In this work, a novel β‐glucosidase (WP_026963033.1) of the glycosyl hydrolase family 1 (GH1) from the extremophilic organism Alicyclobacillus herbarius (Ahe) has been identified and investigated. β‐Glucosidases (EC 3.2.1.21) constitute a group of enzymes that hydrolyse terminal, non‐reducing glycosyl residues from glycosides. AheGH1 is arranged into a single (β/α)8 barrel fold, common to this family of glycosidases, with negligible main‐chain displacements in peripheral loops and α‐helices. As a particular example, the evaluation of the hydrolytic capacity of AheGH1 towards the most common isoflavone glucosides found in soybeans, concluded that the enzyme can efficiently convert isoflavone glucosides into aglycones, and hence, it constitutes a promising candidate for the enzymatic production of soybean isoflavones.

Crystals of AheGH1 enzyme belonging to the monoclinic space group P21 diffracted at 1.98 Å resolution. The asymmetric unit of AheGH1 contains four independent molecules, with a calculated Matthews coefficient of 2.42 Å3 Da1 (estimated solvent content of 49.31 %). The overall structure of the four AheGH1 subunits is identical (RMSD values of 0.05 to 0.08 Å over 356 backbone Cα atoms). Electron density map was overall of good quality, with electron density coverage across residues 2‐450 (chain A), 2‐451 (chain B), 3‐447, (chain C) and 3‐446 (chain D), except for a short stretch (P304‐D322). In addition, two nickel cations were identified in the model, present during the affinity chromatography purification step. The metal cations are located at the dimer interfaces between chain A and the symmetry‐related monomer C and between the B and D subunits and are coordinated in a tetrahedral arrangement by the side chains contributed from two histidine (H61) and two glutamate (E29) residues. The molecular weight was determined to be 99.7 KDa by gel filtration, consistent with it being a dimer in solution. Regions which show more significative changes in the secondary structure correspond to residues 272 to 281, folded into a gamma and two β‐turns, and residues 409 to 416 that form two β‐turns instead of the more common α‐helices. In agreement with CBG and other GH1 members in general, the active site pocket contains several conserved polar and aromatic residues that are typically present in carbohydrate recognition sites that binds the nonreducing end of the substrate. Based on comparisons with GH1 members, AheGH1 the main active site residues present are: R79, H122, E167, N166, N296, Y298, E356 and W402 (Figures 3 and S3+4). Based on comparisons made with GH1 members in general, E167 and E356 are likely to be the acid‐base catalyst and nucleophile, respectively in the reaction.

>MTREFISFPQDFLFGTATASYQIEGAVHEDGRGESIWDRFSHTPGKVYQGHTGDVACDHYHRYREDVALMKELGIPAYRFSIAWPRIFPEKGMKNEAGLDFYRRLLEALHEADIRSFVTLYHWDLPQWLQDRGGWANRDTAEYFAEYASLIYERLGDGIDAFITHNEPWCAAFLGHGFGVHAPGHTDWREAFQAAHHILYSHGLAVQAHRASSHKGQIGITLNFTWVDAATDSATDQAAAEVSHAFNNRWFLEPVAGRGYPQEFQQLVEQRIGQFDFVRQGDLAVIAEPIDFLGINFYTRSVVAANPDDALFGLRTLEAPADNRTEMGWEIHPDSLYRLLTWVQSVTGQLPLYITENGAAFADEPVNGRVEDVRRIHYIADHLEAAKRFVDAGGPLKGYFLWSFMDNFEWALGYSKRFGMVYVDYESQQRLVKDSGRWFSEQIAAHKGQVRA[4x]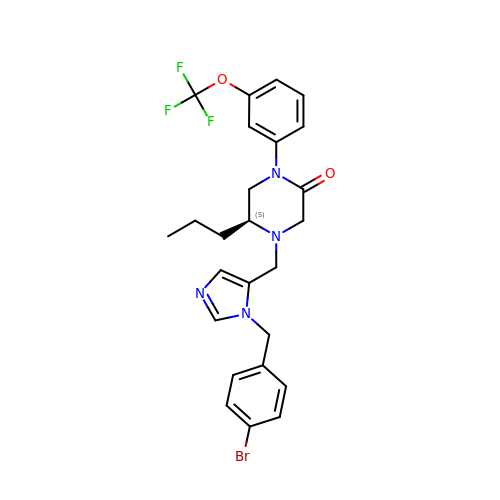(5S)-4-({1-[(4-bromophenyl)methyl]-1H-imidazol-5-yl}methyl)-5-propyl-1-[3-(trifluoromethoxy)phenyl]piperazin-2-one | C25 H26 Br F3 N4 O2 | MMOUEYPUGKAJHU-NRFANRHFSA-N> GAMVQISEVRGNTRDHRTAAHTHIKGLGLNSSGIAEKQAAGFVGQCAAREACGVVVDLIKAHKMAGRGVLLAGGPGTGKTALALAISQELGTKIPFCPITGSEIYSTEVKKTEVLMENFRRAIGLRVRETKDVYEGEVTEMTPEEAENPLGGYGKTISTLLIGLKSARGQKKLRLDPSIYEAIQKERVQVGDVIYIETNTGACKRVGRSDAYATEFDLEAEEYVPIPKGEVHKKKEIVQDVTLHDLDVANARPQGGQDIISMMGQLMKPKMTEITDKLRMEINKVVQKYINQGVAELIPGVLFIDEAHMLDIECFTYLNKALESPIAPIVVLASNRGIATIRGADDLKAAHGIPPDFLQRL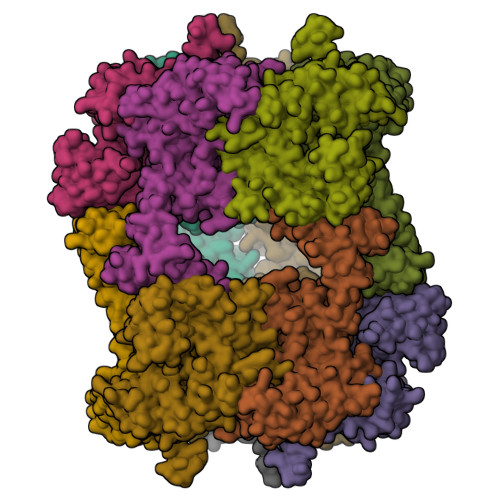LIIPTHPYEPDEIRRIVRIRAQTEGVQLTDAAVDRVAEHGVRISLRYCLQLLAPASILARVNGRTQVDVQDIAEAEELFLDARRSANILTSTGESGGLHGFIS;> GAMAAPLVTSVTETKELRGLNLIAAHSHIRGLGVDADTLEPRPSSQGLVGQEKARKAAAVVLEMIKQGKIAGRAVLIAGPPSTGKTAIAMGMAQSLGQDVPFTTLAASEIFSLEMSKTEALTQAFRKSIGVRIKEESEIMEGEVVEIQIDRSVTGGAKQGKLTIKTTDMEAIYDMGSKMIDAMTKERVMAGDIISIDKSSGKITKLGRSYARSRDYDAMGVDTKFLQCPEGELQKRKEVVHTVSLHEIDVINSRTQGFLALFSGDTGEIRSEIRDQINTKVAEWKEEGKAEIVPGVLFIDEVHMLDIECFSYINRALESDLAPIVIMASNRGVSRIRGTDYKSPHGLPLDFLDRVVIINTHPYTPDELRQILSIRAQEEEVDLTPDALALLTKIGQEAGLRYASNLITTSQLIAAKRRAKQVGVEDVQRSFKLFYDPARSVRFVQESEKRLIGNDGVVDFSYQGAAEAAAPTLPAAAPVDPVGGEKMDMS>GMATVILESIFLKRSQQKKKTSPLNFKKRLFLLTVQKLSYYEYDFERGRRGSKKGSIDVEKITCVETVVPEKNPPPERQIPRRGEESSETEQISIIERFPYPFQVVYDEGPLYVFSPTEELRKRWIHQLKNVIRYNSDLVQKYHP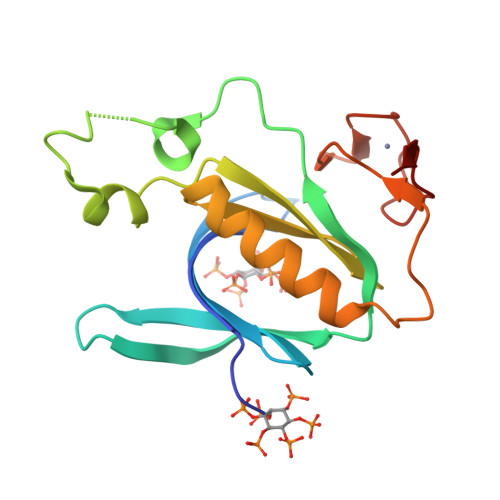CFWIDGQYLCCSQTAKNAMGCQILEN[4x]> PVERILEAELAVEPKTETYVEANMGLNPSSPNDPVTNICQAADKQLFTLVEWAKRIPHFSELPLDDQVILLRAGWNELLIASFSHRSIAVKDGILLATGLHVHRNSAHSAGVGAIFDRVLTELVSKMRDMQM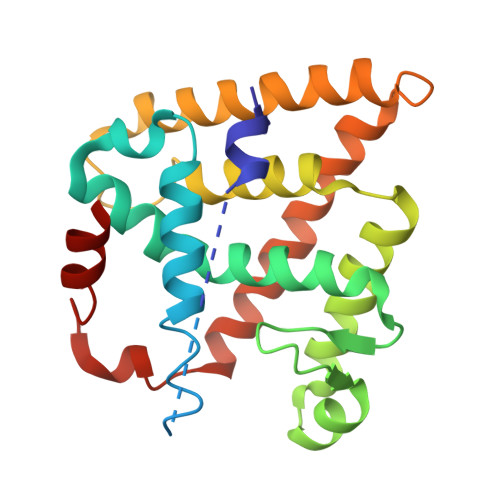DKTELGCLRAIVLFNPDSKGLSNPAEVEALREKVYASLEAYCKHKYPEQPGRFAKLLLRLPALRSIGLKCLEHLFFFKLIGDTPIDTFLMEML>[4x]MLRAAARFGPRLGRRLLSAAATQAVPAPNQQPEVFCNQIFINNEWHDAVSRKTFPTVNPSTGEVICQVAEGDKEDVDKAVKAARAAFQLGSPWRRMDASHRGRLLNRLADLIERDRTYLAALETLDNGKPYVISYLVDLDMVLKCLRYYAGWADKYHGKTIPIDGDFFSYTRHEPVGVCGQIIPWNFPLLMQAWKLGPALATGNVVVMKVAEQTPLTALYVANLIKEAGFPPGVVNIVPGFGPTAGAAIASHEDVDKVAFTGSTEIGRVIQVAAGSSNLKRVTLELGGKSPNIIMSDADMDWAVEQAHFALFFNQGQCCCAGSRTFVQEDIYDEFVERSVARAKSRVVGNPFDSKTEQGPQVDETQFKKILGYINTGKQEGAKLLCGGGIAADRGYFIQPTVFGDVQDGMTIAKEEIFGPVMQILKFKTIEEVVGRANNSTYGLAAAVFTKDLDKANYLSQALQAGTVWVNCYDVFGAQSPFGGYKMSGSGRELGEYGLQAYTEVKTVTVKVPQKNS

Here we report the use of single particle cryo-EM to identify multiple proteins from three enriched heterogeneous fractions prepared from human liver mitochondrial lysate. Using this approach, we were able to simultaneously identify and solve cryo-EM structures of nine different human mitochondrial enzymes: short chain acyl-CoA dehydrogenase (SCAD), medium chain acyl-CoA dehydrogenase (MCAD), isovaleryl-CoA dehydrogenase (IVD), delta (3, 5)-delta dienoyl-CoA isomerase (ECH1), aspartate aminotransferase (GOT2), glutamate dehydrogenase (GLUD1), mitochondrial superoxide dismutase 2 (SOD2), catalase (CAT), and mitochondrial aldehyde dehydrogenase (ALDH2). Functionally, the three acyl-CoA dehydrogenases—SCAD, MCAD and IVD—are involved in beta oxidation and amino acid catabolism. Finally, SOD2, CAT, and ALDH2 are all involved in clearing toxic byproducts of oxidative respiration.

Mitochondrial ALDH is localized in the mitochondrial matrix with a primary role in metabolizing acetaldehyde to acetate in the alcohol metabolism pathway. We collected a total of 82,360 single-particle cryo-EM projections for this class of protein images. Based on these projections, the BaR methodology allowed us to construct a high-resolution cryo-EM map. Subsequently, we were able to identify this protein as the ALDH2 enzyme and resolve its structure to a resolution of 2.66 Å. Matching with existing crystal structures of the ALDH2 enzyme, each ALDH2 subunit consists of a coenzyme domain, a catalytic domain, and an oligomerization domain. The coenzyme domain (24–155 and 176–287) possesses an NADH-binding site. Both the cofactor and catalytic domain (residues 288–502) contain a five stranded α/β sheet followed by two antiparallel β strands. The oligomerization domain (156–175 and 503–511) is a three stranded antiparallel β sheet. Presumably, residues W185, N186, K209, E212, S263, Q366, E285, and C319 are engaged in NADH binding and C319 is the catalytic residue. However, we did not observe bound NADH in our cryo-EM structure.> MHKSAFQALQGDIPTYEVNSSDEQDSDQDEEDVEQPSEPMHRLVSAPAASIHIEESKYISSNFSFDDDNTIYGHDYVIFGLKSNQNLIVKGQFVLEIQRGAIDINGVIYHSGVEPMKFINPSSSSIPLIQATQVLNSSLLENKESQENQHLFTPGYKSVIKLTNLDTHLESIGRVCPLFKNLFWQFDNFFAEDSLRLLDQYELAFSDYTFYPITKPDNTVSVIKHKNWMDVIKSLTELYSNDQSIKVIVIGGKNSGKSTFLRLLVQHMLSPTLQQLPINFMDLDPGQPEYSGTDCISLSKISEVQHGNHLSLTSTDSTQCHYVGFNSPKDQPTRYNLLVEQLVRSYESDGELKHESLLINTPGWIKGYGLELTRTLIERVKPTHVIYLNSGTLGVDIDIPKGTNLIPLQGSFNHSGSRYSSSQLRLLKTMAYFHKIDDFKFDFQPLLFSPPIQVSYGVSTGISALTHLKETGIGMDHLE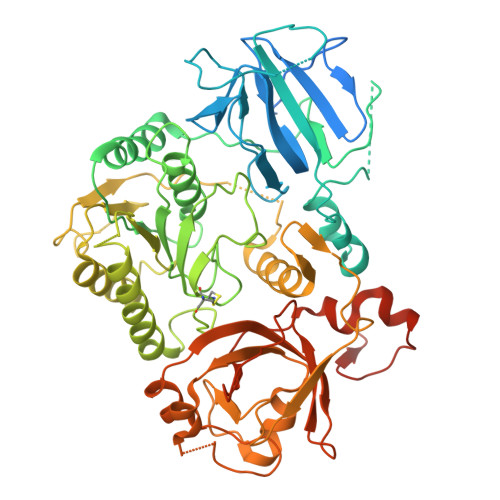RSIEATIVGIFKVKRDHLEECELFNKGQLPLLPYKEFIKLSTEFFRLALVHSIDQEKKIMNLYIPQFRTLDLTKEAIIMVRGNTDLPIWEIASNEIVKRFKRQLPYITFEKGSSLEKKWKVRKNVQRRGQM> MAVPIQKVQDDTKTLIKTIVTRINDISHTQSVSAKQRVTGLDFIPGLHPILSLSKMDQTLAVYQQ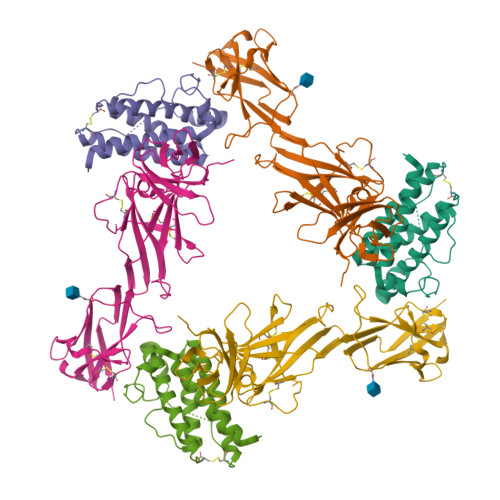VLTSLPSQNVLQIANDLENLRDLLHLLAFSKSCSLPQTSGLQKPESLDGVLEASLYSTEVVALSRLQGSLQDILQQLDVSPEC;> AHHHHHHPGGPGSENLYFQGGSSGTQDVVYFPPKILTSVGSNASFHCIYKNENQIISSKQIVWWRNLAEKIPEIQYSIVSDRVSKVTFSNLKATRPRGKFTYDAVYCCNEQACHHRYAELYVIDVNINISCETDGYLTKMTCRWSPSTIQSLVGSTVQLRYHRRSLYCPDSPSIHPTSEPKNCVLQRDGFYECVFQPIFLLSGYTMWIRINHSLGSLDSPPTCVLPDSVVKPLPPSNVKAEITVNTGLLKVSWEKPVFPENNLQFQIRYGLSGKEIQWKTHEVFDAKSKSASLLVSDLSAVYVVQVRCRRLDGLGYWSNWSSPAYTLVMD> MPVFHTRTIESILEPVAQQISHLVIMHEEGEVDGKAIPDLTAPVAAVQAAVSNLVRVGKETVQTTEDQILKRDMPPAFIKVENACTKLVQAAQMLQSDPYSVPARDYLIDGSRGILSGTSDLLLTFDEAEVRKI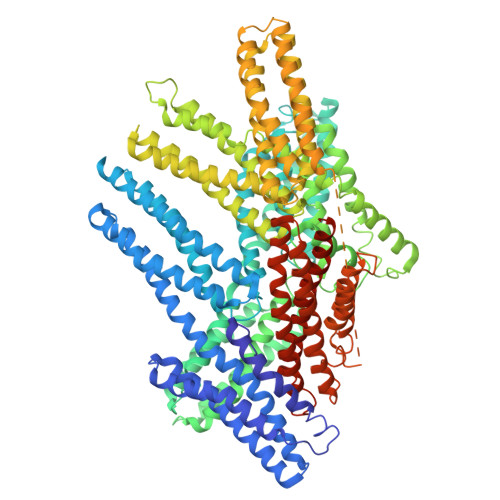IRVCKGILEYLTVAEVVETMEDLVTYTKNLGPGMTKMAKMIDERQQELTHQEHRVMLVNSMNTVKELLPVLISAMKIFVTTKNSKNQGIEEALKNRNFTVEKMSAEINEIIRVLQLTSWDEDAWASKDTEAMKRALASIDSKLNQAKGWLRDPSASPGDAGEQAIRQILDEAGKVGELCAGKERREILGTCKMLGQMTDQVADLRARGQGSSPVAMQKAQQVSQGLDVLTAKVENAARKLEAMTNSKQSIAKKIDAAQNWLADPNGGPEGEEQIRGALAEARKIAELCDDPKERDDILRSLGEISALTSKLADLRRQGKGDSPEARALAKQVATALQNLQTKTNRAVANSRPAKAAVHLEGKIEQAQRWIDNPTVDDRGVGQAAIRGLVAEGHRLANVMMGPYRQDLLAKCDRVDQLTAQLADLAARGEGESPQARALASQLQDSLKDLKARMQEAMTQEVSDVFSDTTTPIKLLAVAATAPPDAPNREEVFDERAANFENHSGKLGATAEKAAAVGTANKSTVEGIQASVKTARELTPQVVSAARILLRNPGNQAAYEHFETMKNQWIDNVEKMTGLVDEAIDTKSLLDASEEAIKKDLDKCKVAMANIQPQMLVAGATSIARRANRILLVAKREVENSEDPKFREAVKAASDELSKTISPMVMDAKAVAGNISDPGLQKSFLDSGYRILGAVAKVREAFQPQEPDFPPPPPDLEQLRLTDELAPPKPPLPEGEVPPPRPPPPEEKDEEFPEQKAGEVINQPMMMAARQLHDEARKWSSKPGIPAAEVGIGVVAEADAADAAGFPVPPDMEDDYEPELLLMPSNQPVNQPILAAAQSLHREATKWSSKGNDIIAAAKRMALLMAEMSRLVRGGSGTKRALIQCAKDIAKASDEVTRLAKEVAKQCTDKRIRTNLLQVCERIPTISTQLKILSTVKATMLGRTNISDEESEQATEMLVHNAQNLMQSVKETVREAEAASIKIRTDAGFTLRWVRKTPWYQHHHHHHHH>GPGSMTDQAAPALKEIFNVERLQHIASEMTAVYPAFDAKGFLKHAKAGLAELSVMQRMARVSESLHAVIPLDYPQTLTLLYALAPRLNSGFVSLFLPHYVASYGRDDFKRSMAALKYFTTFGSAEFAIRHFLLHDFQRTLAVMQAWSQDDNEHVRRLASEGSRPRLPWSFRLAEVQADPELCASILDHLKADSSLYVRKSVANHLNDITKDHPEWVLSLIEGWNLENPHTAWIARHALRSLIKQGNTRALTLMGAGAKAEVKI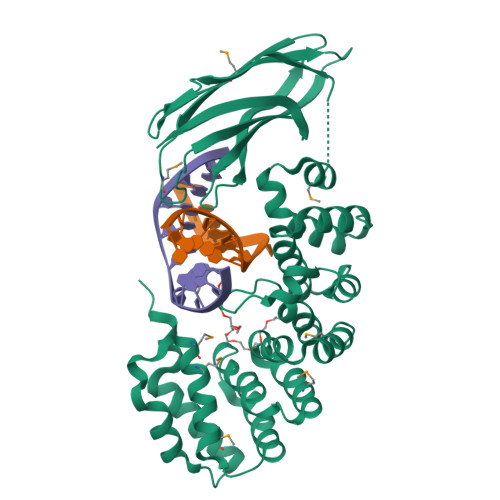HHLMVTPAVINLGERINLSFTLESTAPAPQKLVVDYAIDYVKSTGHGAAKVFKLKAFSLGAGAQQHIRREQHIRDMTTRKHYPGRHVVHVLVNGERLGSAEFELRA[2x]>[2x]GAAAGGGGAGUAGCGUCGGGAAACCG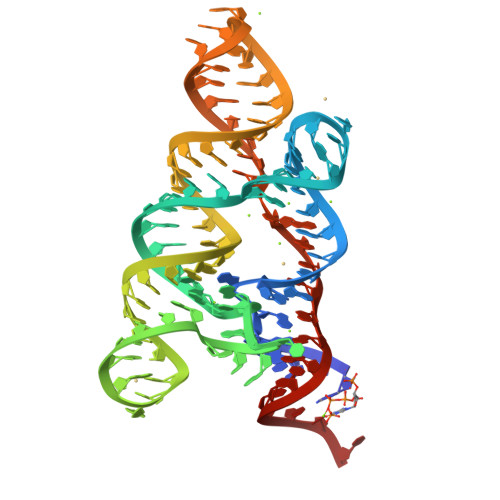AAACAAAGUCGACAUACUGUGAGGAAACUCACCGGCUUUGUUGACAUACGAAAGUAUGUUUAGCAAGACCUUUCC>LEEKKVCQGTSNKLTQLGTFEDHFLSLQRMFNNCEVVLGNLEITYVQRNYDLSFLKTIQEVAGYVLIALNTVERIPLENLQIIRGNMYYENSYALAVLSNYDANKTGLKELPMRNLQEILHGAVRFSNNPALCNVESIQWRDIVSSDFLSNMSMDFQNHLGSCQKCDPSCPNGSCWGAGEENCQKLTKIICAQQCSGRCRGKSPSDCCHNQCAAGCTGPRESDCLVCRKFRDEATCKDTCPPLMLYNPTTYQMDVNPEGKYSFGATCVKKCPRNYVVTDHGSCVRACGADSYEMEEDGVRKCKKCEGPCRKVCNGIGIGEFKDSLSINATNIKHFKNCTSISGDLHILPVAFRGDSFTHTPPLDPQELDILKTVKEITGFLLIQAWPENRTDLHAFENLEIIRGRTKQHGQFSLAVVSLNITSLGLRSLKEISDGDVIISGNKNLCYANTINWKKLFGTSGQKTKIISNRGENSCKATGQVCHALCSPEGCWGPEPRDCVSCRNVSRGRECVDKCNLLEGEPREFVENSECIQCHPECLPQAMNITCTGRGPDNCIQCAHYIDGPHCVKTCPAGVMGENNTLVWKYADAGHVCHLCHPNCTYGCTGPGLEGCPTNGPKIP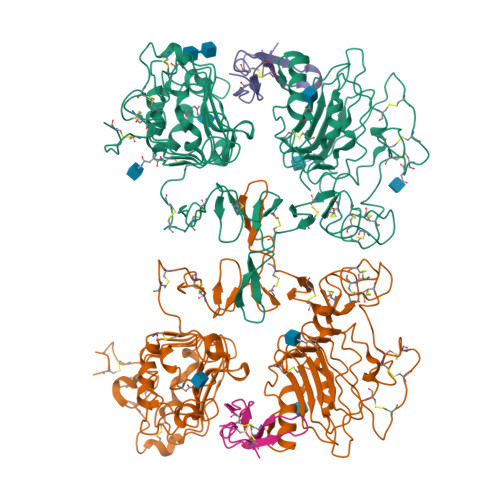SI[2x];>NSDSECPLSHDGYCLHDGVCMYIEALDKYACNCVVGYIGERCQYRDLKWWELR[2x]>MHHHHHHQIGWRREGIKYRRNELFLDVLESVNLLMSPQGQVLSAHVSGRVVMKSYLSGMPECKFGMNDKIVIEKQGKGTADETSKSGKQSIAIDDCTFHQCVRLSKFDSERSISFIPPDGEFELMRYRTTKDIILPFRVIPLVREVGRTKLEVKVVIKSNFKPSLLAQKIEVRIPTPLNTSGVQVICMKGKAKYKASENAIVWKIKRMAGMKESQISAEIELLPTNDKKKWARPPISMNFEVPFAPSGLKVRYLKVFEPKLNYSDHDVIKWVRYIGRSGIYETRC[2x]

Proper operation of the pivotal CME cargo adaptor AP2 requires membrane-localized Fer/Cip4 homology domain-only proteins (FCHO). The AP2 complex, composed of α, β2, μ2, and σ2 subunits, is pivotal to mammalian CCV formation, and its deletion is embryonically lethal in mice. FCHO1 and FCHO2 are similar in overall domain arrangement —folded N-terminal acidic phospholipid-binding homodimerization F-BAR domains and C-terminal folded μ-homology domains (μHD) separated by a ~300-residue, low-complexity intrinsically disordered protein linker, which has been suggested to participate in AP2 activation, although how it does so is undetermined. We dissect the network of interactions between the FCHO interdomain linker and AP2, which concentrates, orients, tethers, and partially destabilizes closed AP2 at the plasma membrane.

To confirm the identity of the extra, Cμ2-proximal electron density as the N terminus of FCHO2 linker, chimeras of Cμ2 alone with N1+N2 attached to the C terminus via 30-residue unstructured synthetic glycine-, serine-, and alanine-rich flexible linkers were then created, crystallized, and their structures solved at resolutions varying from 2.0 to 2.6 Å by MR using an unliganded version of Cμ2 as a search model. Crystals of a complex of Cμ2 and a peptide corresponding to this WxxL signal were grown, diffracted to 1.7-Å resolution, and were solved by MR using 1.9-Å unliganded Cμ2 as a search model.>FVEMVDNLRGKSGQGYYVEMTVGSPPQTLNILVDTGSSNFAVGAAPHPFLHRYYQRQLSSTYRDLRKGVYVPYTQGKWEGELGTDLVSIPHGPNVTVRANIAAITESDKFFINGSNWEGILGLAYAEIARPDDSLEPFFDSLVKQTHVPNLFSLQLCGAGFPLNQSEVLASVGGSMIIGGIDHSLYTGSLWYTPIRREWYYEVIIVRVEINGQDLKMDCKEYNYDKSIVDSGTTNLRLPKKVFEAAVKSIKAASSTEKFPDGFWLGEQLVCWQAGTTPWNIFPVISLYLMGEVTNQSFRITILPQQYLRPVEDVATSQDDCYKFAISQSSTGTVMGAVIMEGFYVVFDRARKRIGFAV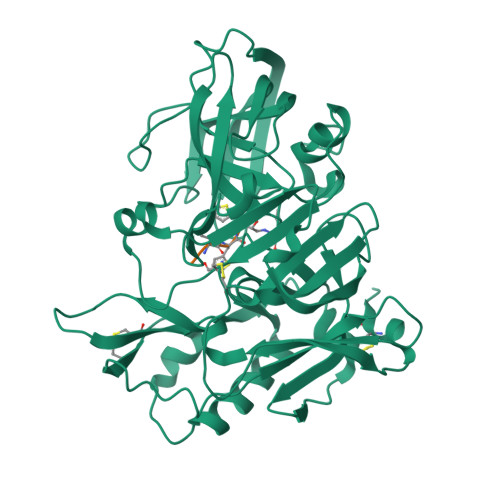SACHVHDEFRTAAVEGPFVTLDMEDCGYNI[3x]> MHHHHHHQIGWRREGIKYRRNELFLDVLESVNLLMSPQGQVLSAHVSGRVVMKSYLSGMPECKFGMNDKIVIEKQGKGTADETSKSGKQSIAIDDCTFHQCVRLSKFDSERSISFIPPDGEFELMRYRTTKDIILPFRVIPLVREVGRTKLEVKVVIKSNFKPSLLAQKIEVRIPTPLNTSGVQVICMKGKAKYKASENAIVWKIKRMAGMKESQISAEIELLPTNDKKKWARPPISMNFEV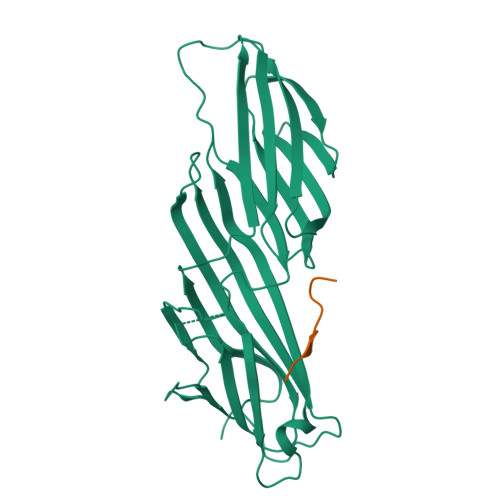PFAPSGLKVRYLKVFEPKLNYSDHDVIKWVRYIGRSGIYETRC;> SHLGTYGVFTNAAFDPSP> MYYGISQFSEAYNKILRNSSSHSSCQLVIFVSCLNIDALCATKMLSLLFKKQLVQSQIVPIFGYSELRRHYSQLDDNINSLLLVGFGGVIDLEAFLEIDPQEYVIDTDEKSGEQSFRRDIYVLDAHRPWNLDNIFGSQIIQCFDDGTVDDTLGEQKEAYYKLLELDEESGDDELSGDENDNNGGDDEATDADEVTDEDEEDEDETISNKRGNSSIGPNDLSKRKQRKKQIHEYEGVLEEYYSQGTTVVNSISAQIYSLLSAIGETNLSNLWLNILGTTSLDIAYAQVYNRLYPLLQDEVKRLTPSSRNSVKTPDTLTLNIQPDYYLFLLRHSSLYDSFYYSNYVNAKLSLWNENGKKRLHKMFARMGIPLSTAQETWLYMDHSIKRELGIIFDKNLDRYGLQDIIRDGFVRTLGYRGSISASEFVEALTALLEVGNSTDKDSVKINNDNNDDTDGEEEEDNSAQKLTNLRKRWVSNFWLSWDALDDRKVELLNRGIQLAQDLQRAIFNTGVAILEKKLIKHLRIYRLCVLQDGPDLDLYRNPLTLLRLGN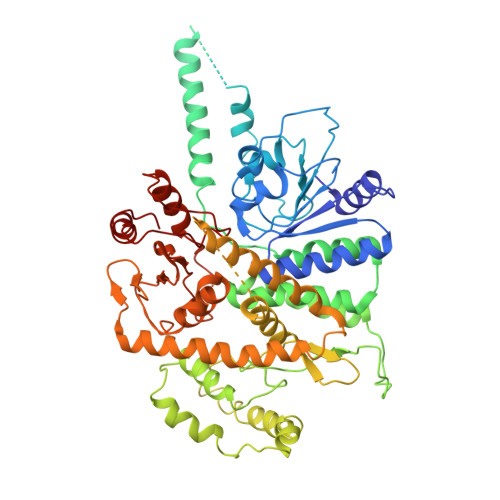WLIECCAESEDKQLLPMVLASIDENTDTYLVAGLTPRYPRGLDTIHTKKPILNNFSMAFQQITAETDAKVRIDNFESSIIEIRREDLSPFLEKLTLSGLL(~{E})-3-[4-oxidanyl-3-[3-(phenylmethyl)phenyl]phenyl]prop-2-enoic 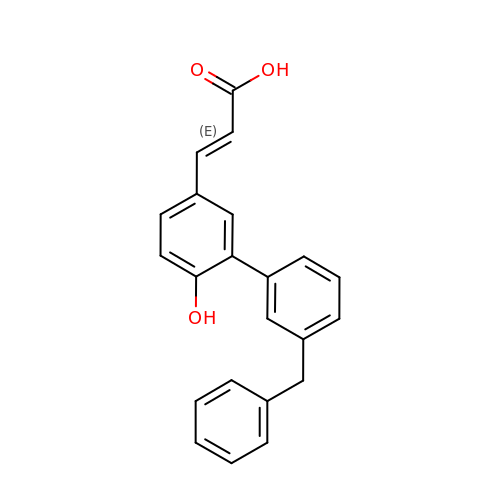acid | C22 H18 O3 | WOWLBKWVURQFNH-ZRDIBKRKSA-N> PGLSCRFYQHKFPEVEDVVMVNVRSIAEMGAYVSLLEYNNIEGMILLSELSRRRIRSINKLIRIGRNECVVVIRVDKEKGYIDLSKRRVSPEEAIKCEDKFTKSKTVYSILRHVAEVLEYTKDEQLESLFQRTAWVF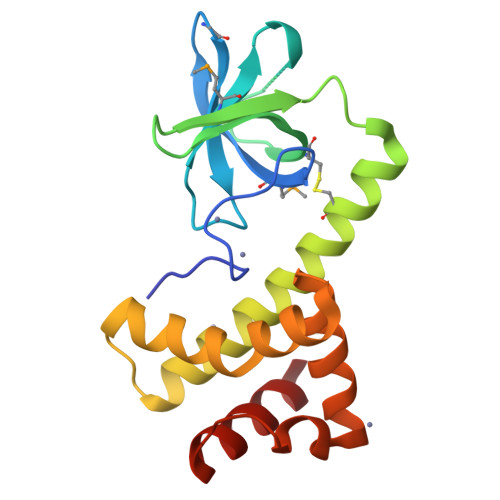DDKYKRPGYGAYDAFKHAVSDPSILDSLDLNEDEREVLINNINRR Previously reported as putative ion channels sensitive to osmolality, a companion paper characterizes OSCA/TMEM63 family members as a novel family of MA ion channels conserved across eukaryotes. The structure of OSCA1.2 reveals a trapezoid-shaped homodimer with a two-fold symmetry axis perpendicular to the membrane. The bulk of the protein lies within the membrane; the transmembrane (TM) domain (TMD) of each monomer contains eleven TM helices. Topological similarities with mTMEM16A suggest that OSCA1.2 also has two pores and could conduct ions through a structurally analogous pathway lined by TM3-TM7.

We purified Arabidopsis thaliana OSCA1.2 expressed in HEK293F cells and determined cryo-EM reconstructions in lipidic nanodiscs and Lauryl Maltose Neopentyl Glycol (LMNG) detergent micelle with cholesteryl hemisuccinate (CHS) at 3.1 and 3.5 Å resolution, respectively. Structures of OSCA1.2 in nanodisc and LMNG were nearly identical (RMSD = 0.81 Å). A comparison of nanodisc-embedded and LMNG-solubilized structures hints at the positional flexibility of the subunits relative to each other while in the closed state. We refer to the nanodisc structure throughout unless otherwise noted because of superior resolution and map quality. The ICD contributes the sole dimeric interface in OSCA1.2, with a buried surface area of 1,331 Å2, only 4% of the total surface area of the dimer. Within the membrane, inter-subunit contacts are nonexistent. Instead, a cleft with minimum width of approximately 8 Å separates one subunit’s TMD from the other. To visualize the dimensions of the putative ion permeation pathway, we used the HOLE program. Towards the extracellular side, this putative pore has an opening greater than 12 Å wide, which narrows into a ‘neck’ approximately 15 Å down the conduction pathway. The neck extends for over 10 Å and reaches a minimum van der Waals radius of 0.5 Å, closing the channel.

>MATLQDIGVSAGINILSAFVFFIIFAVLRLQPFNDRVYFSKWYLKGLRSSPARGGAFAQRFVNLDFRSYMKFLNWMPEALKMPEPELIDHAGLDSVVYLRIYWLGLKIFTPIAVLAWAVLVPVNWTNNTLEMAKQLRNVTSSDIDKLSVSNIPEYSMRFWTHIVMAYAFTIWTCYVLMKEYETIANMRLQFVASEARRPDQFTVLVRNVPPDADESVSELVEHFFLVNHPDHYLTHQVVCNANKLADLVKKKKKLQNWLDYYQLKYARNNSQRIMVKLGFLGLWGQKVDAIEHYIAEIDKISKEISKEREEVVNDPKAIMPAAFVSFKTRWAAAVCAQTQQTRNPTQWLTEWAPEPRDVFWSNLAIPYVSLTVRRLIMHVAFFFLTFFFIVPIAFVQSLATIEGIVKAAPFLKFIVDDKFMKSVIQGFLPGIALKLFLAFLPSILMIMSKFEGFTSISSLERRAAFRYYIFNLVNVFLASVIAGAAFEQLNSFLNQSANQIPKTIGVAIPMKATFFITYIMVDGWAGVAGEILMLKPLIMFHLKNAFLVKTDKDREEAMDPGSIGFNTGEPRIQLYFLLGLVYAPVTPMLLPFILVFFALAYIVYRHQIINVYNQEYESAAAFWPDVHGRVIAALVISQLLLMGLLGTKHAALAAPFLIALPVLTIGFHHFCKGRYEPAFIRYPLQEAMMKDTLETAREPNLNLKGYLQNAYVHPVFKGDEDDYDIDDKLGKFEDEAIIVPTKRQSRRNTPAPSIISGDDSPSLPFSGKLVGTGTLEVLFQ[2x]> AH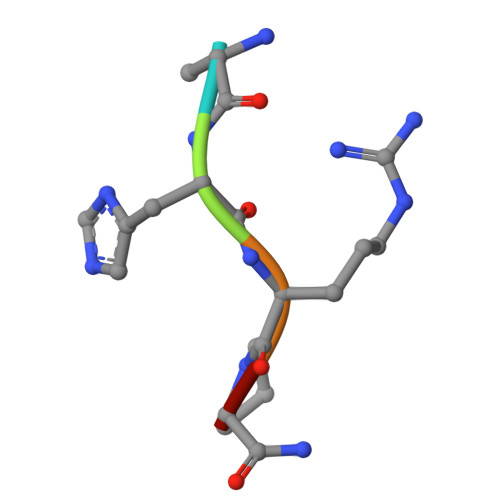RPX>[4x]MESRYVLTGRYDSAPATDGSG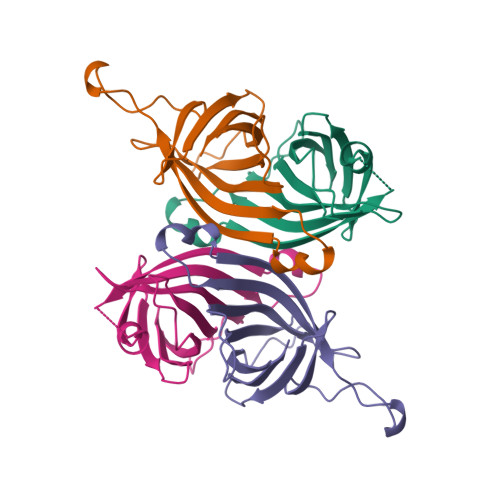TALGWTVAWKNNYRNAHSATTWSGQYVGGAEARINTQWLLTSGTTEANAWKSTLVGHDTFTKVKPSAASGGGSAEAGITGTWYNQLGSTFIVTAGADGALTGTYESA> MKHQHQHQHQHQHQQPLQEEEQAHATSLPPRASSPPQILPQLSPEQLGMIEKLVAAQQQCNRRSFSDRLRVTPWPM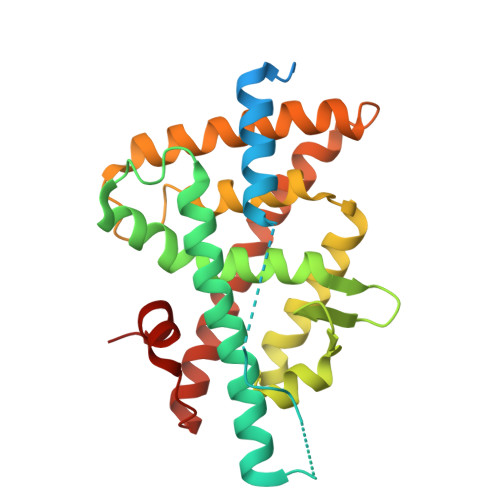APDPHSREARQQRFAHFTELAIVSVQEIVDFAKQLPGFLQLSREDQIALLKTSAIEVMLLETSRRYNPGSESITFLKDFSYNREDFAKAGLQVEFINPIFEFSRAMNELQLNDAEFALLIAISIFSADRPNVQDQLQVERLQHTYVEALHAYVSIHHPHDRLMFPRMLMKLVSLRTLSSVHSEQVFALRLQDKKLPPLLSEIWDVHE(2~{S})-~{N}-(3,5-dimethylphenyl)-1-(4-methoxyphenyl)sulfonyl-pyrrolidine-2-carboxamide 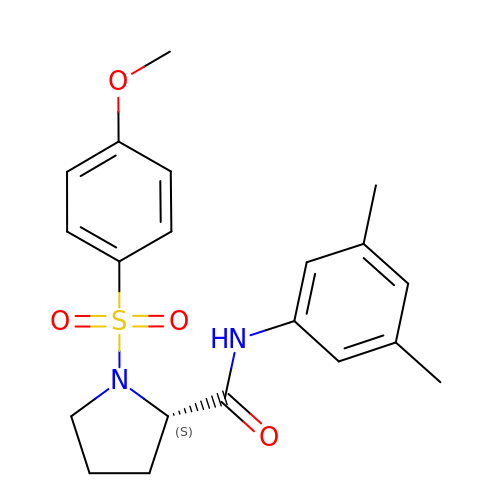| C20 H24 N2 O4 S | NHPQGZOBHSVTAQ-IBGZPJMESA-N>[2x]MTTPPLLQLPVEVKKTELNGFWDTGAQITCIPEAFLKEEIPIGEAQIKTLHGTKLQSVYYLKFKVLGRKVEAEVTTSPFDYVIISPSDIPWYKPQPLELTVKLPVQDFKKELINKANINNEEKKQLAKLLDKYDVLWQQWENQVGHRKIPPHNIATGTVAPRPQRQYHINTKAKPSIQQVIDDLLKQGVLIKQTSVMNTPIYPVPKPDGKWRMVLDYRAVNKTVPLIGAQNQHSLGILTNLVRQKYKSTIDLSNGFWAHPITKDSQWITAFTWEGKQHVWTRLPQGFLNSPALFTADVVDLLKNIPGISVYVDDIYFSTETVSEHLKILEKVFKILLEAGYIVSLKKSALLRYEVTFLGFSITQTGRGLTSEFKDKIQNITSPRTLKELQSILGLFNFARNFVPNFSEIIKPLYSLISTAEGNNIKWTSEHTRYLEEIVSALNHAGNLEQRDNESPLVVKLNASPKTGYIRYYNKGGQKPIAYASHVFTNTELKFTPLEKLLVTMHKALIKAIDLALGQPIEVYSPIISMQKLQKTPLPERKALSTRWITWLSYLEDPRITFYYDKTLPDLKNVPETVTDKKPKMLPII

Reverse transcriptases (RTs) use their DNA polymerase and RNase H activities to catalyze the conversion of single-stranded RNA to double-stranded DNA (dsDNA), a crucial process for the replication of retroviruses. Foamy viruses (FVs) have many characteristics that set them apart from OVs, including differences in the proliferation cycle and a different domain structure of the mature RT, which, in addition to POL and RH, harbors the N-terminal protease (PR) domain (PR-RT). Reverse transcriptases have two activities: DNA polymerase (POL) synthesizes DNA on DNA or RNA templates, whereas RNase H (RH) degrades the RNA strand of RNA/DNA hybrid intermediates. The structural and biophysical experiments showed that MFV PR-RT is a monomer upon binding to RNA/DNA and a dimer when it interacts with dsDNA.

The second crystal form was obtained using a deletion variant of MFV PR-RT that lacked the RH domain (MFV PR-RT ΔRH) and was grown in the presence of 13-bp dsDNA with a 5′ overhang of 2 nt in one strand (substrate 2) (see Materials and Methods for the sequence). Unexpectedly, the complete model of MFV PR-RT ΔRH revealed a dimer of the protein that interacted with the dsDNA duplex. One subunit that we termed subunit A adopts a structure that is analogous to the monomeric form that is observed in the full-length MFV PR-RT hybrid complex structure (RMSD of 2.6 Å over 477 Cα atoms), with small differences in the positions of the individual (sub)domains. However, the conformation of the other subunit (subunit B) is markedly different. The palm/finger module remains largely the same, but the position of the finger/thumb module is completely rearranged such that it blocks the POL active site. This conformation is very similar to the ones that were observed for the p51 subunit of HIV-1 RT and subunit B of Ty3 RT, with the largest differences in the positioning of the thumb subdomain. Similar to other RT structures, the recessed 3′ end of the DNA interacts with the POL active site of subunit A. The PR domains of both subunits are also visible in the structure. Interestingly, they interact with each other. However, the dimeric arrangement of the PR domains in our structure is markedly different from the architecture of stand-alone PRs such as the HIV-1 enzyme and would not allow active-site formation. In the PR-RT ΔRH structure, protein-dsDNA interactions are observed along almost the entire length of the nucleic acid, and these contacts are mostly mediated by subunit A of the dimer.> GDQMISHRELWAKIANSINDINEQYLKVYEHAVSSYTQMYQDFSAVLSSLAGWISPGGNDGNSVKLQVNSLKKALEELKEKYKDKPLYPANNTVSQEQANKWLTELGGTIGKVSQK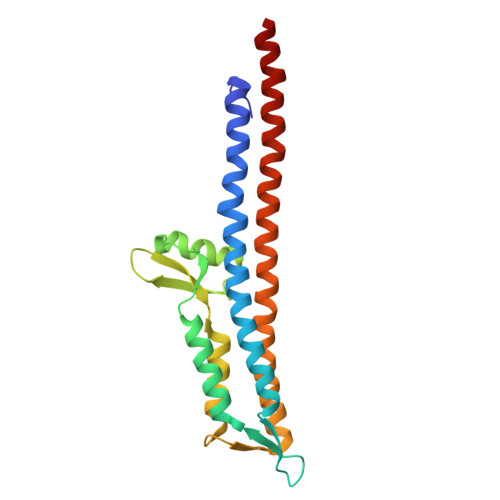NGGYVVSINMTPIDNMLKSLDNLGGNGEVVLDNAKYQAWNAGFSAEDETMKNNLQTLVQKYSNANSIFDNLVKVLSSTISSCTDTDKLFLHF>GMAKVKIVGILNVTPNSFHDGGRFVETDKAVVRARELLSQGADIIEIGGESTGPGSNTITADEELARIVPVIRAIRSSLPDANIAVDTYKAEVARKALELGATMINDVSAGRADPKLFGVVARSNAQIVLMYSKDTDPHTSFDERQYVDVVRTVYDFLAERKKAAM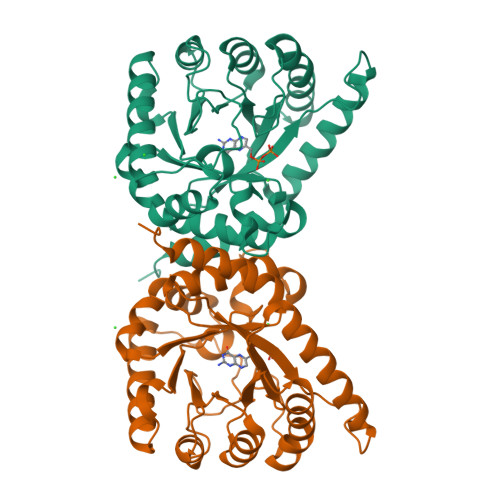SAGIPADRIILDTGLGHFVSSDPQYSFQLLAHLSDFQDLGCKLFLSPSRKSFLAGNELLKTADRLPGTIAASAIAVLHGADYIRTHDVLEVRRGCEIATAINQPPER[2x]> MPLLTQQIQDEDDQYSLVASLDNVRNLSTILKAIHFREHATCFATKNGIKVTVENAKCVQANAAIQAGIFQEFKVQEESVTFRINLTVLLDCLSIFGSSPMPGTLTALRMCYQGYGYPLMLFLEEGGVVTVCKINTQEPEETLDFDFCSTNVINKIILQSEGLREAFSELDMTSEVLQITMSPDKPYFRLSTFGNAGSS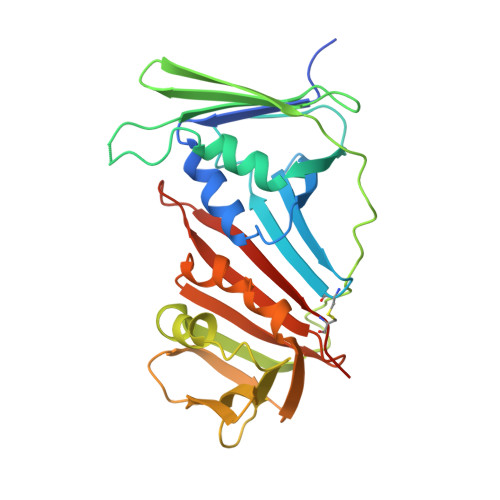HLDYPKDSDLMEAFHCNQTQVNRYKISLLKPSTKALVLSCKVSIRTDNRGFLSLQYAIRNEDGQICAVEYYCCPDEEVPESES>AESLPDLKIEKLDEGVYVHTSFEEVNGWGVVPKHGLVVLVNAEAYLIDTPFTAKDTEKLVTWFVERGYKIKGSISSHFHSDSTGGIEWLNSRSIPTYASELTNELLKKDGKVQATNSFSGVNYWLVKNKIEVFYPGPGHTPDNVVVWLPERKILFGGCFIKPYGLGNLGDANIEAWPKSAKLLKSKYGKAKLVVPGHSEVGDASL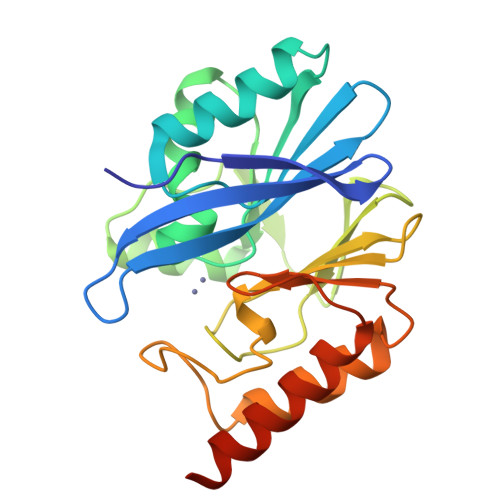LKLTLEQAVKGLNESKKPSKPSN[4x]>[2x]ISHMSSHHHHHHIQNRAQAVDQLRAVARYFRQTEPHSPVAYLADKAA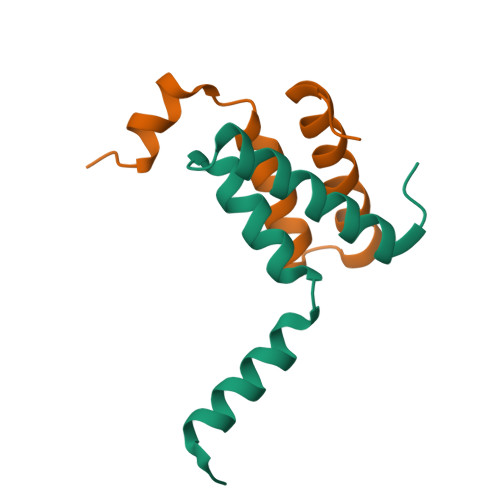EWADMPLHKWLESVVKDDGSL>GIGTGFPFDPHYVEVLGERMHYVDVGPRDGTPVLFLHGNPTSSYVWRNIIPHVAPTHRCIAPDLIGMGKSDK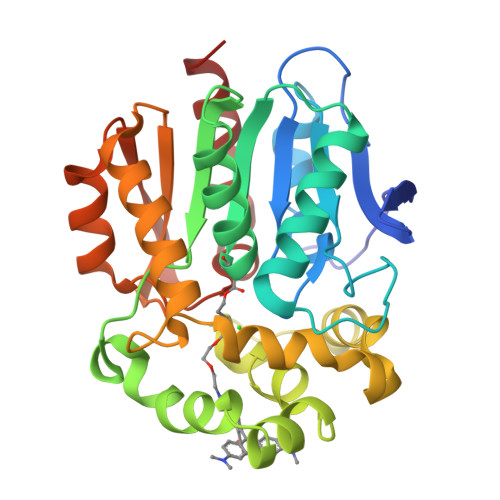PDLGYFFDDHVRFMDAFIEALGLEEVVLVIHDWGSALGFHWAKRNPERVKGIAFMEFIRPIPTWDEWPEFARETFQAFRTTDVGRKLIIDQNVFIEGTLPWGVVRPLTEVEMDHYREPFLNPVDREPLWRFPNELPIAGEPANIVALVEEYMDWLHQSPVPKLLFWGTPGVLIPPAEAARLAKSLPNCKAVDIGPGLNLLQEDNPDLIGSEIARWLSTLEI[4x]>ISSCNGPCRDLNDCDGQLICIKGKCNDDPEVGTHICRGT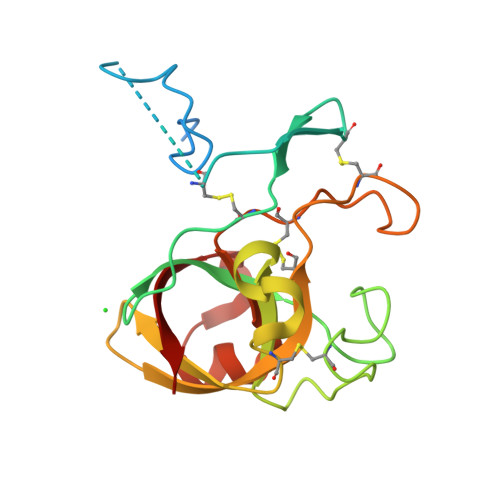TPSPQPGGCKPSGTLTCQGKSHPTYDCSPPVTSSTPAKLTNNDFSEGGDGGGPSECDESYHSNNERIVALSTGWYNGGSRCGKMIRITASNGKSVSAKVVDECDSRHGCDKEHAGQPPCRNNIVDGSNAVWSALGLNKNVGVVDITWSMA[2x]>[2x]MSDKDSKNTPQVPEKLGLSRRGFLGASAVTGAAVAATALGGAVMTRESWAQAVKESKQKIHVGPGELDDYYGFWSGGHQGEVRVLGVPSMRELMRIPVFNVDSATGWGLTNESRHIMGDSAKFLNGDCHHPHISMTDGKYDGKYLFINDKANSRVARIRLDIMKCDKMITVPNVQAIHGLRLQKVPHTKYVFANAEFIIPHPNDGKVFDLQDENSYTMYNAIDAETMEMAFQVIVDGNLDNTDADYTGRFAAATCYNSEKAFDLGGMMRNERDWVVVFDIHAVEAAVKAGDFITLGDSKTPVLDGRKKDGKDSKFTRYVPVPKNPHGCNTSSDGKYFIAAGKLSPTCSMIAIDKLPDLFAGKLADPRDVIVGEPELGLGPLHTTFDGRGNAYTTLFIDSQVVKWNMEEAVRAYKGEKVNYIKQKLDVHYQPGHLHASLCETNEADGKWLVALSKFSKDRF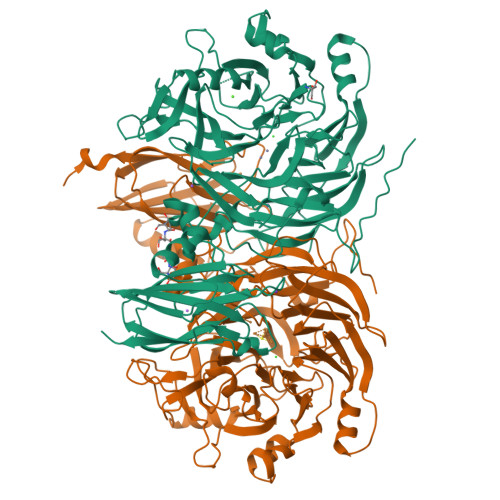LPVGPLHPENDQLIDISGDEMKLVHDGPTFAEPHDCIMARRDQIKTKKIWDRNDPFFAPTVEMAKKDGINLDTDNKVIRDGNKVRVYMTSMAPAFGVQEFTVKQGDEVTVTITNIAQIEDVSYGFVVVNHGVSMEISPQQTSSITFVADKPGLHWYYCSWFCHALHMEMVGRMMVEPAWSHPQFEK>MKKIEHKMVAVNGLNMHLAELGEGPTILFIHGFPELWYSWRHQMVYLAERGYRAVAPDLRGYGDTTGAPLNDPSKFSILHLVGDVVALLEAIALNEEKVFVVA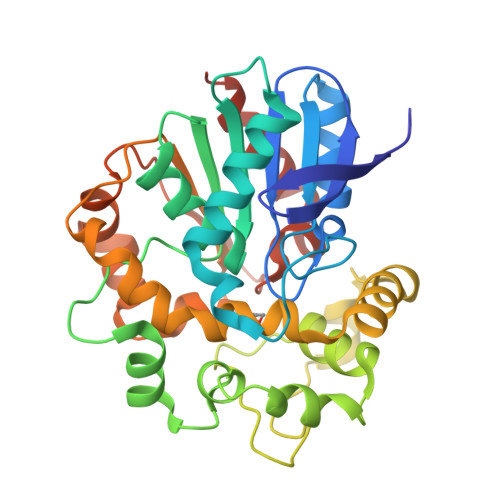HDLGAYIAWHLCLFRPDKVKALVNLSVHFSKRNPKMNKVEGLKAIYGEDHYVSRFQVPGEIEAEFAPIGAKSVLKKILTYRDPAPFYFPKGKGLEAIPDAPVALSSWLSEEELDYYANKFEQTGFTGAVNYYRALPINWELTAPWTGAQVKVPTKFIVGEFDLVYHIPGAKEYIHNGGFKKDVPLLEEVVVLEGAAHFVSQERPHEISKHIYDFIQKFTSHHHHH[2x]>[2x]MDSKYQCVKLNDGHFMPVLGFGTYAPAEVPKSKALEAVKLAIEAGFHHIDSAHVYNNEEQVGLAIRSKIADGSVKREDIFYTSKLWSNSHRPELVRPALERSLKNLQLDYVDLYLIHFPVSVKPGEEVIPKDENGKILFDTVDLCATWEAMEKCKDAGLAKSIGVSNFNHRLLEMILNKPGLKYKPVCNQVECHPYFNQRKLLDFCKSKDIVLVAYSALGSHREEPWVDPNSPVLLEDPVLCALA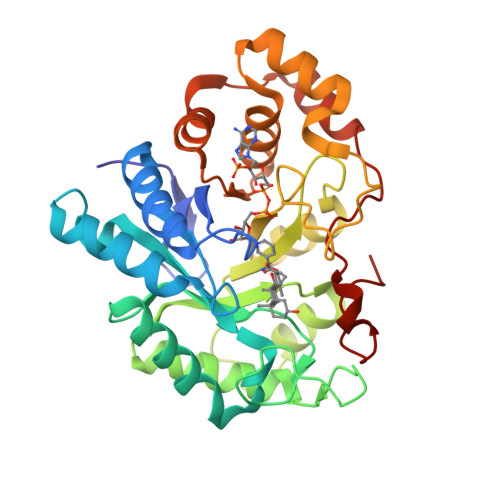KKHKRTPALIALRYQLQRGVVVLAKSYNEQRIRQNVQVFEFQLTSEEMKAIDGLNRNVRYLTLDIFAGPPNYPFSDEY>[2x]GSHMSEQFDFDLERILKTIKDKNCK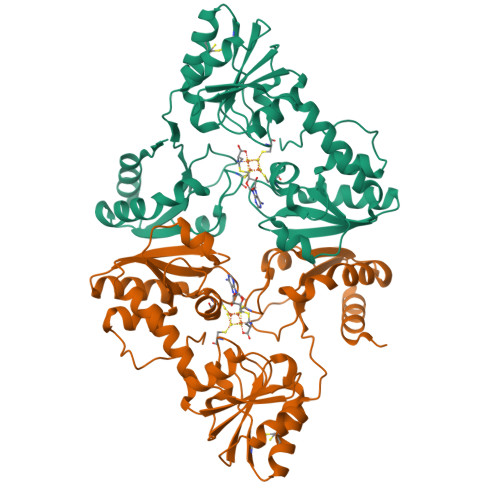KVGLQFPEGLKRQAINIAREIEEKTRANVIISGNPCFGACDIDTILAGSVDILFHFGHAGMGEYENVVFIEARSNIDIIPAVKTALNLLKANRIGLITTVQHVHKLEEACKVIKEYGKECVIGKGDPRAIYPGQVLGCNFTAARVDCEEFIYIGSGIFHPLGVAIATKKRVIAADPFLNQAVEVSPERFLRKRGGYIAKATGAKIFGIIVSTKSGQYRMKLAQKLKEIADKHGKIGYIILMDLVTPEQLLAFKADAYVNTACPRITIDDAERFHAPVLTPQEFEIVLGERRWENMEMDEMIQ> MPMYEDRIDLYGADGKLLEEDVPLEAISPLKNPTIANLVSDVKRSVAVNLAGIEGSLRKAALGGKSNFIPGREVELPIVENAEAIAEKVKKLVQTSEDDDTNIRLINNGQQILVQVPTTRMGVAADYTVSALVTGAAVVQAIIDEFDVDMFDANAVKTAVMGRYPQTVDFTGANLSTLLGPPVLLEGLGYGLRNIMANHVVAITRKNTLNASALSSILEQTAMFETGDAVGAFERMHLLGLAYQGLNANNLLFDLVKENGKGTVGTVIASLVERAVEDGVVKVAREMNSGYKVYEPADWALW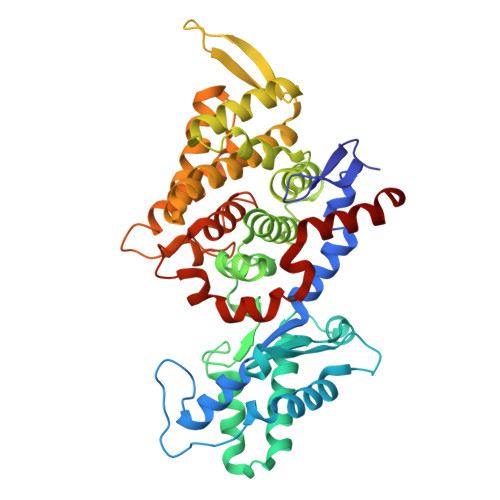NAYAATGLLAATIVNVGAARAAQGVASTVLYYNDILEYETGLPGVDFGRAMGTAVGFSFFSHSIYGGGGPGIFHGNHVVTRHSKGFALPCVAAAMCLDAGTQMFSVEKTSGLIGSVYSEIDYFREPIVNVAKGAAEVKDQL> GDPIADMIDQTVNNQVNRSLTALQVLPTAANTEASSHRLGTGVVPALQAAETGASSNASDKNLIETRCVLNHHSTQETAIGNFFSRAGLVSIITMPTTGTQNTDGYVNWDIDLMGYAQLRRKCELFTYMRFDAEFTFVVAKPNGELVPQLLQYMYVPPGAPKPTSRDSFAWQTATNPSVFVKMTDPPAQVSVPFMSPASAYQWFYDGYPTFGEHLQANDLDYGQCPNNMMGTFSIRTVGIEKSPHSITLRVYMRIKHVRAWIPRPLRNQPYLFKTNPNYKGNDIKCTSTSRDKITTL;> SPSAEACGYSDRVAQLTIGNSTITTQEAANIVIAYGEWPEYCPDTDATAVDKPTRPDVSVNRFFTLDTKSWAKDSKGWYWKFPDVLTEVGVFGQNAQFHYLYRSGFCVHVQCNASKFHQGALLVAVLPEYVLGTIAGGTGNENSHPPYATTQPGQVGAVLTHPYVLDAGIPLSQLTVCPHQWINLRTNNCATIIVPYMNTVP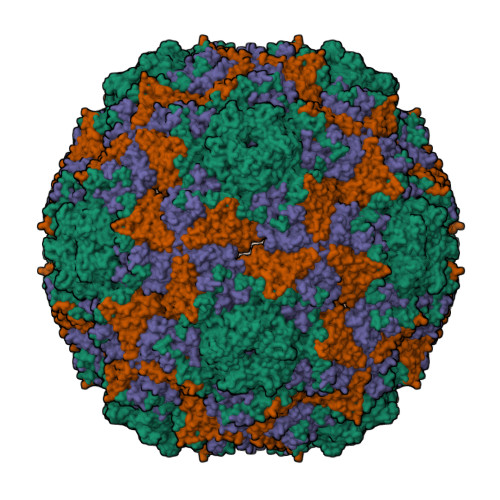FDSALNHCNFGLLVIPVVPLDFNTGATSEIPITVTIAPMCAEFAGLRQAVKQ;> GIPTELKPGTNQFLTTDDGVSAPILPGFHPTPPIHIPGEVHNLLEICRVETILEVNNLKTNETTPMQRLCFPVSVQSKTGELCAAFRADPGRDGPWQSTILGQLCRYYTQWSGSLEVTFMFAGSFMATGKMLIAYTPPGGNVPADRITAMLGTHVIWDFGLQSSVTLVVPWISNTHYRAHARAGYFDYYTTGIITIWYQTNYVVPIGAPTTAYIVALAAAQDNFTMKLCKDTEDIEQTANIQ>[2x]MGSSHHHHHHSQDPNSSSARLQVEMGDKFGEGRDPYLYPGLDIMRNRLNIHQQQRLEQAAYEMTALRAATIELGPLVRRLPHLRTIHRQLYQDIFDWAGQLREVDIYQGDTPFCHFAYIEKEGNALMQDLEEEGYLVGLEKAKFVERLAHYYCEINVLHPFRVGSGLAQRIFFEQLAIHAGYQLSWQGIEKEAWNQAN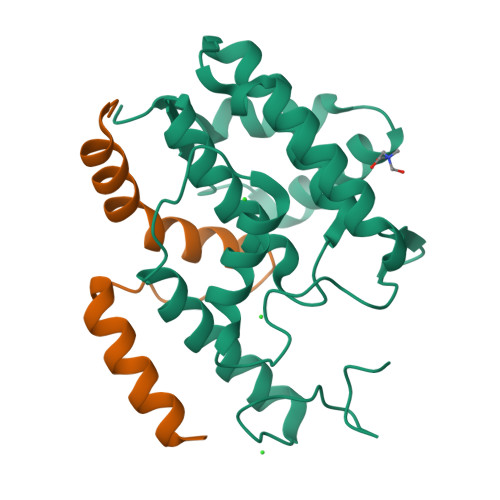QSGAMGDLTALQMIFSKVVSEAGESE;>MAYPYDVPDYAAAVKKLTDKQKSRLWELQRNRNFQASRRLEGVEMPLVTLTAAEALARLEELRSHYER[2x]>MTQCYAEITGWGKCLPPATLSNHDLSTFLDTSDEWIQSRTGIEQRRISHVNTSDLATVAAQHAIACAGVSVEEIDLIIVATCSPDSLIPNIASRVQQNLGIPSAAAFDLNAAATGFLYGLETATRLMQASHYRHALVIGAERLSFYLDWTKRDTAVLFGDGAGAVVLSKTEQKVGLQDAQIGCDAQGRDILAVPKFGT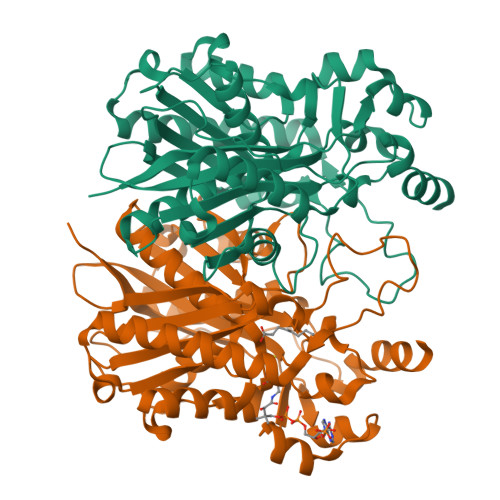AMDRFDADNGYWAFDFVGKEIFKRAVRGMGAAAQQVLARSGLSTEEIDVVIPHQANIRIIQTLCDLAGIAQDKAFVNIHRYGNTSAATVPIALCEALEQGKIKPHDDLLVAAFGAGLTWGAGHIRWGERITPLGKSDAQLPSCDHTALDLLSKAIEHCKRHQSE[2x]>[4x]STPPPLNFSRASEHRNEKGERISMINPRVVLDENGISHRSRYFIMLCDNETAIAHAKKTSIWAVKKDSSKRISDAYKKASVYFIFVAQQTYNALGYAQVVS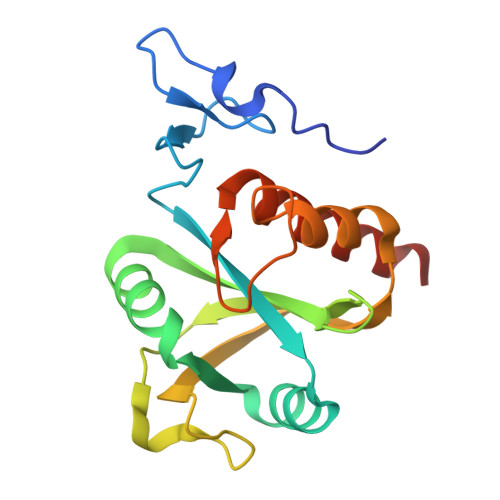DLNSTELPFWSDSSHAGGVRIKWIKTCNLFSAEISEIVSHMDHGSEARDGMEMMYDEGSRLCTLINYAIMKRIGRDR ADENOSINE-5'-TETRAPHOSPHATE | C10 H17 N5 O16 P4 | 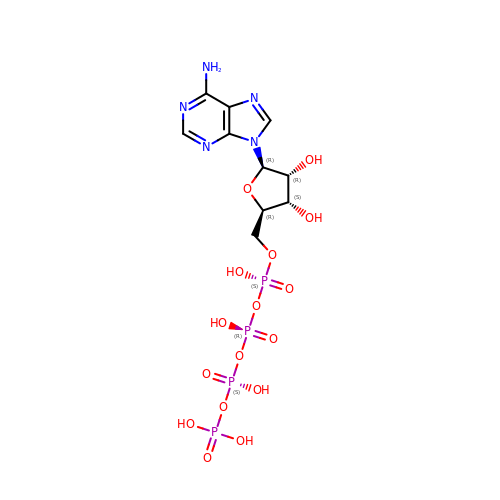WWMWAMFHUSTZTA-KQYNXXCUSA-N>[4x]MQEIALTPQPAHLTVKDGRFEFGNQLKAKVTPYQGDSIRMVFESFKKELQEATGIKVSSTQKEAKARIILDL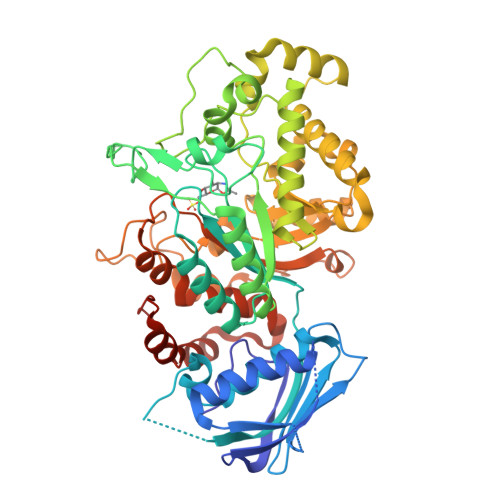NPQLPAEAYKLNVSKKQVRIEASRPAGFYYALQTLKQLMPRNVMAGVATSDHSQWSLPSVEIEDAPRFEWRGFMLDEGRHFFGKDEIKRVIDMMAIYKMNRFHWHLTEDQGWRIEIKKYPKLTETGAWRNSKVLAYGDVKPDGERYGGFYTQKDIKEIVAYAKKKFIEIIPEIDIPGHSQAAVAAYPEFLACDPRDKHEVWLQQGISTDVINVANPKAMQFAKEVIDELTELFPFNYIHLGGNECPTRKWQKNDECKKLLSEIGSSNFRDLQIYFYKQLKDYIATKPADQQRQLIFWNEVLHGNTSILGNDITIMAWIGANAAAKQAAKQGMNTILSPQIPYYINRKQSKLPTEPMSQGHGTETVEAVYNYQPLKDVDAALQPYYKGVQANFWTEWVTEPSVLEYLMLPRLAAVAEAGWTPQEKRNYEDFKERIRKDAELYDLKGWNYGKHIMKLEHHHHHH>ENLMQVYQQARLSNPELRKSAADRDAAFEKINEARSPLLPQLGLGADYTYSNGYRDANGINSNATSASLQLTQSIFDMSKWRALTLQEKAAGIQDVTYQTDQQTLILNTATAYFNVLNAIDVLSYTQAQKEAIYRQLDQTTQRFNVGLVAITDVQNARAQYDTVLANELTARNNLDNAVEQLRQITGNYYPELAALNVENFKTDKPQPVNALLKEAEKRNLSLLQARLSQDLAREQIRQAQDGHLPTLDLTASTGISDTSYSGSKTRGAAGTQYDDSNMGQNKVGLSFSLPIYQGGMVNSQVKQAQYNFVGASEQLESAHRSVVQTVRSSFNNINASISSINAYKQAVVSAQSSLDAMEAGYSVGTRTIVDVLDATTTLYNAKQELANARYNYLINQLNIKSALGTLNEQDLLALNNALSKPVSTNPENVAPQTPEQNAIADGYAPDSPAPVVQQTSARTTTSNGHNPFRNDYKDDDDK[3x];>MKKRKTVKKRYVIALVIVIAGLITLWRILNAPVPTYQTLIVRPGDLQQSVLATGKLDALRKVDVGAQVSGQLKTLSVAIGDKVKKDQLLGVIDPEQAENQIKEVEATLMELRAQRQQAEAELKLARVTYSRQQRLAQTQAVSQQDLDNAATEMAVKQAQIGTIDAQIKRNQASLDTAKTNLDYTRIVAPMAGEVTQITTLQGQTVIAAQQAPNILTLADMSAMLVKAQVSEADVIHLKPGQKAWFTVLGDQLTRYEGQIKDVLPTPEKVNDAIFYYARFEVPNPNGLLRLDMTAQVHIQLTDVKNVLTIPLSALGDPVGDNRYKVKLLRNGETREREVTIGARNDTDVEIVKGLEAGDEVVIGEAKPGAAQ[6x];>MTPLLELKDIRRSYPAGDEQVEVLKGISLDIYAGEMVAIVGASGSGKSTLMNILGCLDKATSGTYRVAGQDVATLDADALAQLRREHFGFIFQRYHLLSHLTAEQNVEVPAVYAGLERKQRLLRAQELLQRLGLEDRTEYYPAQLSGGQQQRVSIARALMNGGQVILADEPTGALDSHSGEEVMAI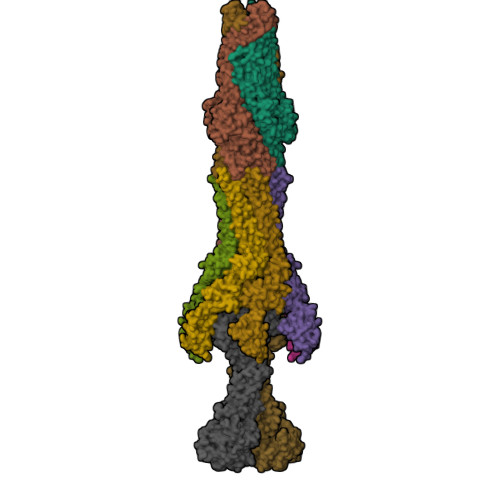LHQLRDRGHTVIIVTHDPQVAAQAERVIEIRDGEIVRNPPAIEKVNVTGGTEPVVNTVSGWRQFVSGFNEALTMAWRALAANKMRTLLTMLGIIIGIASVVSIVVVGDAAKQMVLADIRSIGTNTIDVYPGKDFGDDDPQYQQALKYDDLIAIQKQPWVASATPAVSQNLRLRYNNVDVAASANGVSGDYFNVYGMTFSEGNTFNQEQLNGRAQVVVLDSNTRRQLFPHKADVVGEVILVGNMPARVIGVAEEKQSMFGSSKVLRVWLPYSTMSGRVMGQSWLNSITVRVKEGFDSAEAEQQLTRLLSLRHGKKDFFTWNMDGVLKTVEKTTRTLQLFLTLVAVISLVVGGIGVMNIMLVSVTERTREIGIRMAVGARASDVLQQFLIEAVLVCLVGGALGITLSLLIAFTLQLFLPGWEIGFSPLALLLAFLCSTVTGILFGWLPARNAARLDPVDALAREHHHHHH[2x]> MFERFTDRARRVVVLAQEEARMLNHNYIGTEHILLGLIHEGEGVAAKSLESLGISLEGVRSQVEEIIGQGQQAPSGHIPFTPRAK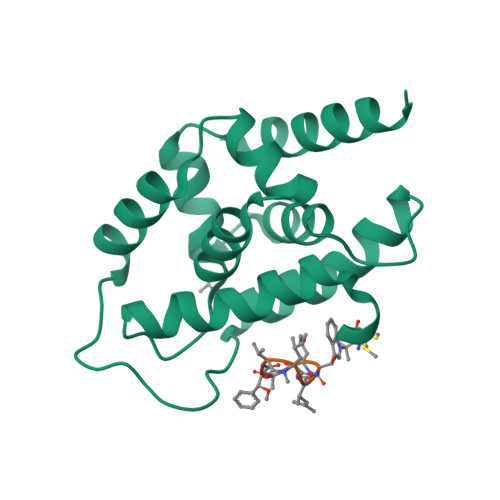KVLELSLREALQLGHNYIGTEHILLGLIREGEGVAAQVLVKLGAELTRVRQQVIQLLSGYLEHHHHHH;> WLAFVLV> GSMSKIYHHPVQIYYEDTDHSGVVYHPNFLKYFERAREHVIDSDKLATLWNDHGLGFAVYKANMIFQDGVEFAEICDIRTSFTLDGKYKTLWRQEVWRPGASR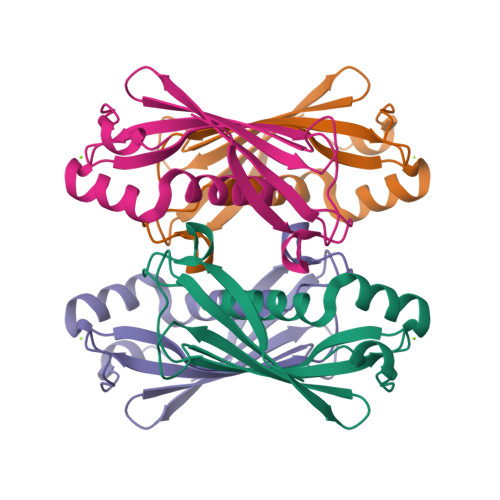AAVIGDIEMVCLDKEKRLQPVPADILASMMAD>[2x]PSVYDAAA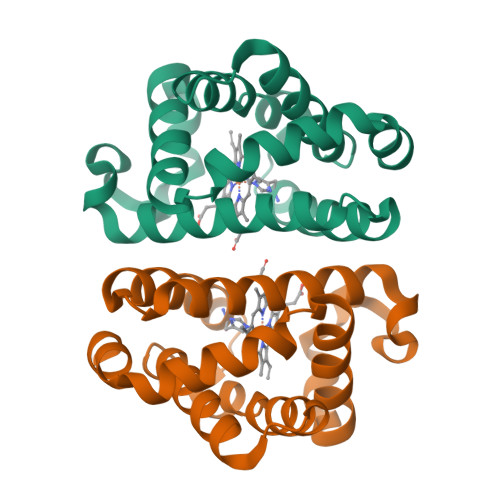QLTADVKKDLRDSWKVIGSDKKGNGVALMTTLFADNQETIGYFKRLGDVSQGMANDKLRGHSITLMYALQNFIDQLDNPDDLVCVVEKVAVNHITRKISAAEFGKINGPIKKVLASKNFGDKYANAWAKLVAVVQAAL> MRPYTLSVALPGSILDNAQSPELRTYLAGQIARACAIFCVDEIVVFDEEGQDAKTVEGEFTGVGKKGQACVQLARILQYLECPQYLRKAFFPKHQDLQFAGLLNPLDSPHHMRQDEESEFREGIVVDRPTRPGHGSFVNCGMKKEVKIDKNLEPGLRVTVRLNQQQHPDCKTYHGKVVSSQDPRTKAGLYWGYTVRLASCLSAVFAEAPFQDGYDLTIGTSERGSDVASAQLPNFRHALVVFGGLQGLEAGADADPNLEVAEPSVLFDLYVNTCPGQGSRTIRTEENILISLAALQPGLIQAGARHT

SPOUT1, also known as CENP-32 or C9ORF114, contains a putative SpoU-TrmD (SPOUT) RNA methyltransferase (MTase) domain. SPOUT1/CENP-32 localized to mitotic spindles and kinetochores, and its depletion by siRNA resulted in unusual centrosome detachment from the mitotic spindle poles, delayed anaphase onset, and chromosome segregation errors. Structural analysis confirmed that SPOUT1/CENP-32 is a SPOUT MTase with a trefoil knot fold consisting of parallel six stranded β-sheets sandwiched between two layers of α-helices that promote dimerization of the protein. Our SPOUT1/CENP-32 structures also reveal that SPOUT1/CENP-32 dimerizes via a helical segment in the catalytic domain that packs almost perpendicularly against an equivalent segment from its dimeric counterpart.

To assess if the observed activity is specific and depends on SPOUT1/CENP-32’s ability to bind its cofactor SAM, we mutated Ala356, an amino acid residue located at the centre of the SAM binding pocket, to Asn (an amino acid residue with a relatively longer side chain; A356N) and characterized this variant by determining its crystal structure and by subjecting it in our MTase activity assay. The crystal structure of SPOUT1/CENP-32 A356N determined at 2.5 Å resolution, showed that while this variant does not affect the overall structure or the conformation of SAM binding pocket, the variant protein failed to stably bind SAH in the expression host (E. coli), confirming the perturbation of cofactor binding. We tested the SPOUT1/CENP-32 A356N variant in our MTase activity assays and observed that this variant shows reduced activity, indicating that the specific catalytic activity of SPOUT1/CENP-32 depends on cofactor binding. We tested the A356N catalytic variant in our siRNA rescue assays to check whether the methyltransferase activity of SPOUT1/CENP-32 is necessary for its function. Depletion of SPOUT1/CENP-32 and induction of SPOUT1/CENP32 A356N-GFP expression in our stable cell lines failed to rescue the centrosome detachment and micronucleus formation phenotype. Thus, SPOUT1/CENP-32 methyltransferase activity is required for maintaining spindle integrity. As expected, we also observed reduced cell viability for cells expressing SPOUT1/CENP32 catalytic variant (SPOUT1/CENP32 A356N-GFP) with reduced methyltransferase activity. These data together indicate that the role of SPOUT1/CENP-32 in regulating spindle organization is dependent on its methyltransferase activity.>MSSKPKPIEIIGAPFSKGQPRGGVEKGPAALRKAGLVEKLKETEYNVRDHGDLAFVDVPNDSPFQIVKNPRSVGKANEQLAAVVAETQKNGTISVVLGGDNSMAIGSISGHARVHPDLCVIWVDAHTDINTPLTTSSGNLHGQPVAFLLKELKGKFPDVPGFSWVTPCISAKDIVYIGLRDVDPGEHYIIKTLGIKYFSMTEVDKLGIGKVMEETFSYLLGRKKRPIHLSFDVDGLDPVFTPATGTPVVGGLSYREGLYITEEIYKTGLLSGLDIMEVNPTLGK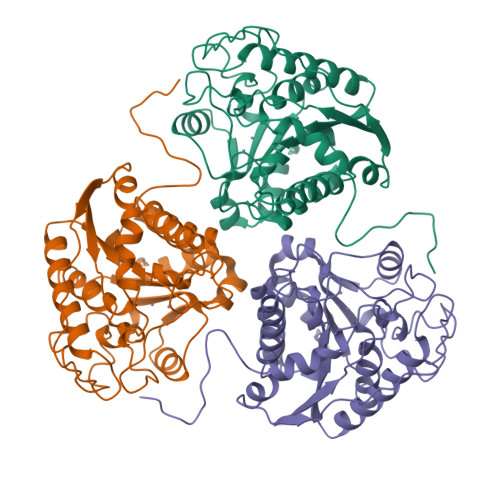TPEEVTRTVNTAVALTLSCFGTKREGNHKPETDYLKPPK[3x]>GRSAMTSVRCKLAQYLEDLEDVDLKKFKMHLEDYPPEKGCIPVPRGQMEKADHLDLATLMIDFNGEEKAWAMAVWIFAAINRRDLWEKAKKDQPEWNDTCTSHSSMVCQEDSLEEEWMGLLGYLSRISICKKKKDYCKMYRRHVRSRFYSIKDRNARLGESVDLNSRYTQLQLVKEHPSKQEREHELLTIGRTKMRDSPMSSLKLELLFEPEDGHSEPVHTVVFQGAAGIGKTILARKIMLDWALGKLFKDKFDYLFFIHCREVSLRTPRSLADLIVSCWPDPNPPVCKILRKPSRILFLMDGFDELQGAFDEHIGEVCTDWQKAVRGDILLSSLIRKKLLPKASLLITTRPVALEKLQHLLDHPRHVEILGFSEAKRKEYFFKYFSNELQAREAFRLIQENEVLFTMCFIPLVCWIV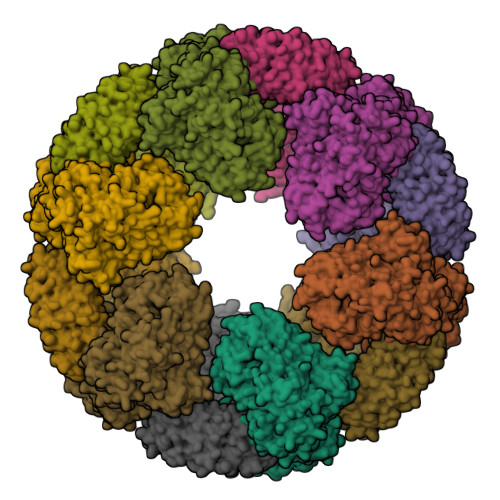CTGLKQQMETGKSLAQTSKTTTAVYVFFLSSLLQSRGGIEEHLFSDYLQGLCSLAADGIWNQKILFEECDLRKHGLQKTDVSAFLRMNVFQKEVDCERFYSFSHMTFQEFFAAMYYLLEEEAEGETVRKGPGGCSDLLNRDVKVLLENYGKFEKGYLIFVVRFLFGLVNQERTSYLEKKLSCKISQQVRLELLKWIEVKAKAKKLQWQPSQLELFYCLYEMQEEDFVQSAMDHFPKIEINLSTRMDHVVSSFCIKNCHRVKTLSLGFFHNSPKEEEEERRGGRPLDQVQCVFPDTHVACSSRLVNCCLTSSFCRGLFSSLSTNRSLTELDLSDNTLGDPGMRVLCEALQHPGCNIQRLWLGRCGLSHQCCFDISSVLSSSQKLVELDLSDNALGDFGIRLLCVGLKHLLCNLQKLWLVSCCLTSACCQDLALVLSSNHSLTRLYIGENALGDSGVQVLCEKMKDPQCNLQKLGLVNSGLTSICCSALTSVLKTNQNFTHLYLRSNALGDTGLRLLCEGLLHPDCKLQMLELDNCSLTSHSCWNLSTILTHNHSLRKLNLGNNDLGDLCVVTLCEVLKQQGCLLQSLQLGEMYLNRETKRALEALQEEKPELTIVFEISW[12x]>MLSRSRCASRAFSRSLSAFQKGNCPLVRRSLPGISLCQGPGYPDSRKTVINSSNIFSVRFFRTTAVCKDDVITVKTPAFAESVTEGDVRWEKAVGDTVAEDEVVCEIETDKTSVQVPSPANGVIEALLVPDGGKVEGGTPLFTLRKTGAAPAKAKPAAAPAAAAPKAEPTVSAVPPPPAAPIPTQMPPVPSPSQPLTSKPVSAVKPTAAPPRAEAGAGVGLRSEHREKMNRMRQRIAQRLKEAQNTCAMLTTFNEIDMSNIQEMRARHKDAFLKKHNLKLGFMSAFVKASAFALQEQPVVNAVIDDATKEVVYRDYIDISVAVATPRGLVVPVIRNVETMNYADIERTISELGEKARKNELAIEDMDGGTFTISNGGVFGSLFGTPIINPPQSAILGMHAIVDRPVVIGGKVEVRPMMYVALTYDHRLIDGREAVTFLRKIKAAVEDPRVLLLDL[24x]

The α-keto acid dehydrogenase complex family catalyzes the essential oxidative decarboxylation of α-keto acids to yield acyl-CoA and NADH. PDC, OGDC, and BCKDC are each comprised of multiple copies of a substrate-specific dihydrolipoamide acetyltransferase (E2p), dihydrolipoamide succinyltransferase (E2o), or dihydrolipoamide acyltransferase (E2b) inner catalytic (IC) core surrounded by multiple copies of the respective α-keto acid dehydrogenase (E1p, E1o, or E1b) and universal dihydrolipoamide dehydrogenase (E3) components. Here, we report the cryo-electron microscopy structures of the endogenous cubic 2-oxoglutarate dehydrogenase complex (OGDC) and icosahedral pyruvate dehydrogenase complex (PDC) cores from bovine kidney determined at resolutions of 3.5 Å and 3.8 Å, respectively. In addition, despite sharing a similar monomeric fold, OGDC and PDC E2 cores have distinct interdomain and intertrimer interactions, which suggests a means of modulating self-assembly to mitigate heterologous binding between mismatched E2 species.

After fitting and real-space refinement of the model into our cubic cryo-EM density map, the side chains for the E2o model fit the density well. The unambiguous identification of the cubic complex as OGDC is further reflected in the low presence of BCKDC components in the mass spectrometry data. For E2o, the backbones of residues 220–455 are fully traceable. The longer βC–βD turn in E2o enables an electrostatic interaction between the negatively charged surface of the turn and the positively charged surfaces of the N-terminus that is not present in E2p. Notably, in bovine E2o, the delocalized π-electron network is extended within the threefold axis and encompasses Phe253, Phe383, and Tyr419. In E2o, H2 has a length of 18 residues (Ser259–His276) and is comprised of a helix–kink–helix with the kink starting at residue 268. The H2 kink in E2o positions the C-terminal end of the helix more closely against H7* for hydrogen bonds between Lys275 and His276 with Asp454* and Asp454*, respectively. In contrast, the E2o knob has an additional hydrophobic surface on the opposite side of the knob, and the E2o socket contains two pockets to accommodate this difference. The exterior of the E2o socket is more charged than that of E2p, which leads to the greater number of hydrogen bonds at the E2o intertrimer interface. The E2o cryo-EM density map also contains a putative lipoyl moiety density.> MNVQLKKQLAELALAGTGH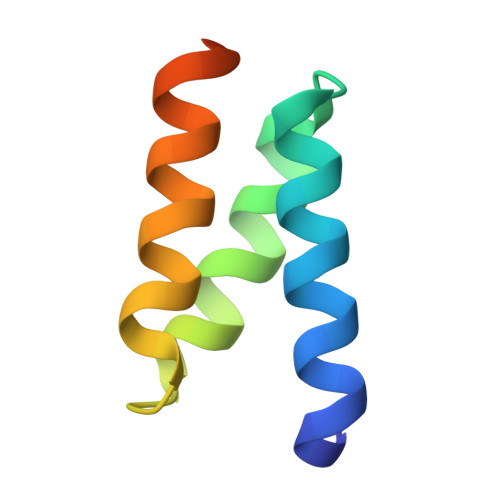HCHQEAASIADWLAQEECMAECVTLIRLSSLMNQGDYQRALL>TCGGTACCG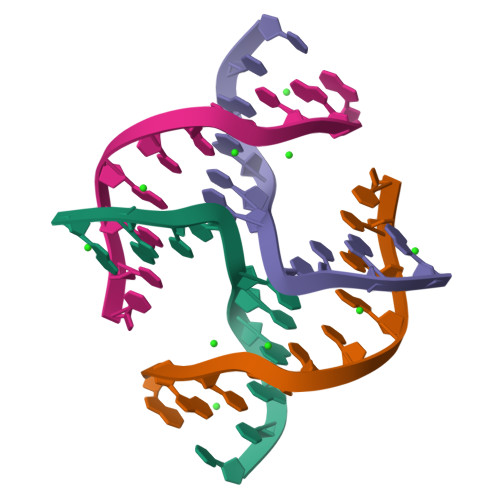A[2x]>MIIREATVQDYYEVARLHTQVHEAHVKERGDIFRSNEPTLNPSRFQAAVQGEKSTVLVFVDEREKIGAYSVIHLVQTPLLPTMQQRKTVYISDLCVDETRRGGGIGRLIFEAIISYGKAHQVDAIEL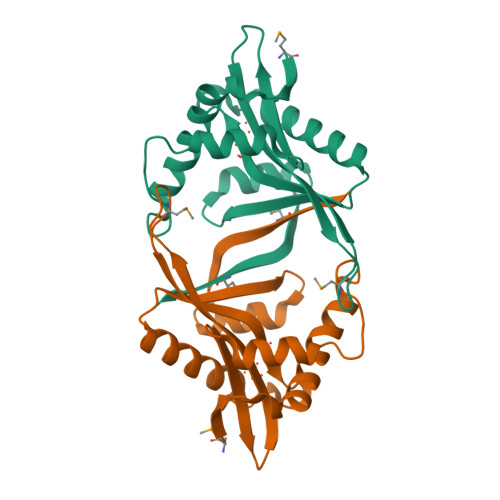DVYDFNERAKRFYHSLGMRCQKQTMELPL[2x]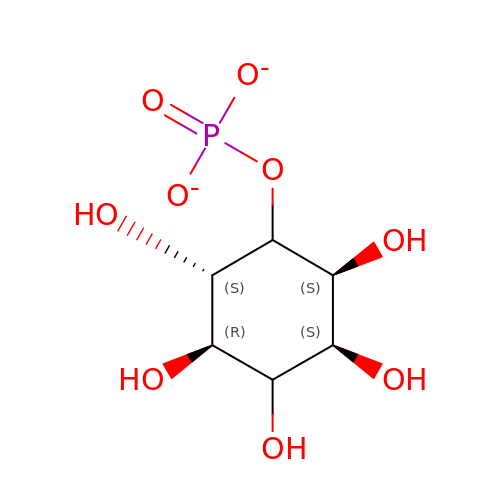L-MYO-INOSITOL-1-PHOSPHATE | C6 H11 O9 P | INAPMGSXUVUWAF-PTQMNWPWSA-L> MAAFVVSTPKKLQTDELATVRLFQENTPSVVYITNLAVRQDAFTLDVLEVPQGSGSGFVWDKQGHIVTNYHVIRGASDLRVTLADQTTFDAKVVGFDQDKDVAVLRIDAPKNKLRPIPVGVSADLLVGQKVFAIGNPFGLDHTLTTGVISGLRREISSAATGRPIQDVIQTDAAINPGNSGGPLLDSSGTLIGINTAIYSPSGASSGVGFSIPVDTVGGIVDQLVRFGKVTRPILGIKFAPDQSVEQLGVSGVLVLDAPPSGPAGKAGLQSTKRDGYGRLVLGDIITSVNGTKVSNGSDLYRILDQCKVGDEVTVE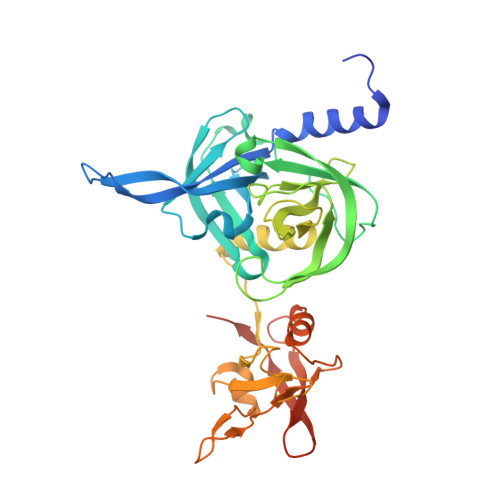VLRGDHKEKISVTLEPKPDESAAALEHHHHHH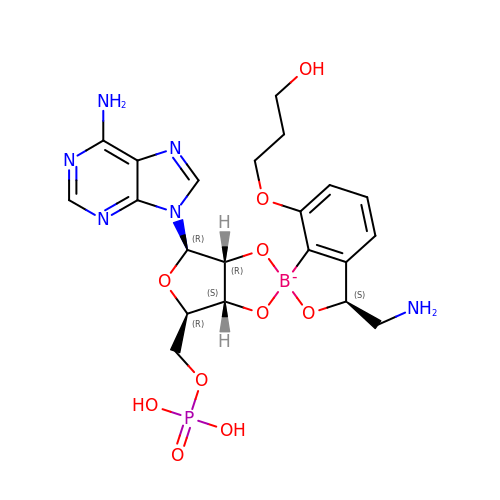[(1S,5R,6R,7'S,8R)-7'-(aminomethyl)-6-(6-aminopurin-9-yl)-2'-(3-oxidanylpropoxy)spiro[2,4,7-trioxa-3-boranuidabicyclo[3.3.0]octane-3,9'-8-oxa-9-boranuidabicyclo[4.3.0]nona-1(6),2,4-triene]-8-yl]methyl dihydrogen phosphate | C21 H27 B N6 O10 P | SQCWYVPZBCHHDX-ZKDXOGESSA-L> MSQFSKDQVQDMYYLSPMQEGMLFHAILNPGQSFYLEQITMKVKGSLNIKCLEESMNVIMDRYDVFRTVFIHEKVKRPVQVVLKKRQFHIEEIDLTHLTGSEQTAKINEYKEQDKIRGFDLTRDIPMRAAIFKKAEESFEWVWSYHHIILDGWCFGIVVQDLFKVYNALREQKPYSLPPVKPYKDYIKWLEKQDKQASLRYWREYLEGFEGQTTFAEQRKKQKDGYEPKELLFSPSEAETKAFTELAKSQHTTLSTALQAVWSVLISRYQQSGDLAFGTVVSGRPAEIKGVEHMVGLFINVVPRRVKLSEGITFNGLLKRLQEQSLQSEPHQYVPLYDIQSQADQPKLIDHIIVFENYPLQDAKNEESSENGFDMVDVHVFEKSNYDLNLMASPGDEMLIKLAYNENVFDEAFILRLKSQLLTAIQQLIQNPDQPVSTINLVDDREREFLLTGLNPPAQAHETKPLTYWFKEAVNANPDAPALTYSGQTLSYRELDEEANRIARRLQKHGAGKGSVVALYTKRSLELVIGILGVLKAGAAYLPVDPKLPEDRISYMLADSAAACLLTHQEMKEQAAELPYTGTTLFIDDQTRFEEQASDPATAIDPNDPAYIMYTSGTTGKPKGNITTHANIQGLVKHVDYMAFSDQDTFLSVSNYAFDAFTFDFYASMLNAARLIIADEHTLLDTERLTDLILQENVNVMFATTALFNLLTDAGEDWMKGLRCILFGGERASVPHVRKALRIMGPGKLINCYGPTEGTVFATAHVVHDLPDSISSLPIGKPISNASVYILNEQSQLQPFGAVGELCISGMGVSKGYVNRADLTKEKFIENPFKPGETLYRTGDLARWLPDGTIEYAGRIDDQVKIRGHRIELEEIEKQLQEYPGVKDAVVVADRHESGDASINAYLVNRTQLSAEDVKAHLKKQLPAYMVPQTFTFLDELPLTTNGKVNKRLLPKPDQDQLAEEWIGPRNEMEETIAQIWSEVLGRKQIGIHDDFFALGGHALKAMTAASRIKKELGIDLPVKLLFEAPTIAGISAYLKNGGSDGLQDVTIMNQDQEQIIFAFPPVLGYGLMYQNLSSRLPSYKLCAFDFIEEEDRLDRYADLIQKLQPEGPLTLFGYSAGCSLAFEAAKKL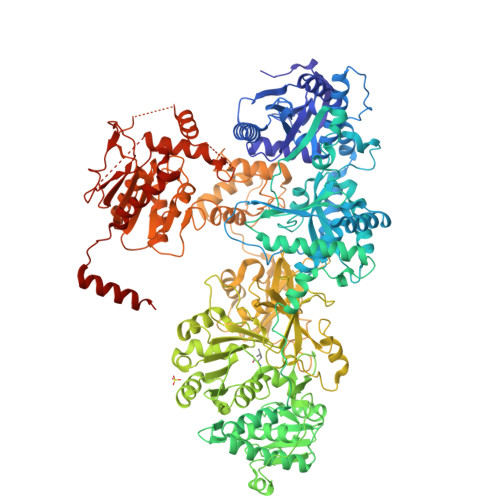EEQGRIVQRIIMVDSYKKQGVSDLDGRTVESDVEALMNVNRDNEALNSEAVKHGLKQKTHAFYSYYVNLISTGQVKADIDLLTSGADFDIPEWLASWEEATTGVYRMKRGFGTHAEMLQGETLDRNAEILLEFLNTQTVTVSKGEFEAYVEQKLISEEDLNSAVDHHHHHH> MAHHHHHHHHHHGSTSGSGEQKLISEEDLGSTSGSGDYKDDDDKLTSLYKKAGLENLYFQGMESEMLQSPLLGLGEEDEADLTDWNLPLAFMKKRHCEKIEGSKSLAQSWRMKDRMKTVSVALVLCLNVGVDPPDVVKTTPCARLECWIDPLSMGPQKALETIGANLQKQYENWQPRARYKQSLDPTVDEVKKLCTSLRRNAKEERVLFHYNGHGVPRPTVNGEVWVFNKNYTQYIPLSIYDLQTWMGSPSIFVYDCSNAGLIVKSFKQFALQREQELEVAAINPNHPLAQMPLPPSMKNCIQLAACEATELLPMIPDLPADLFTSCLTTPIKIALRWFCMQKCVSLVPGVTLDLIEKIPGRLNDRRTPLGELNWIFTAITDTIAWNVLPRDLFQKLFRQDLLVASLFRNFLLAERIMRSYNCTPVSSPRLPPTYMHAMWQAWDLAVDICLSQLPTIIEEGTAFRHSPFFAEQLTAFQVWLTMGVENRNPPEQLPIVLQVLLSQVHRLRALDLLGRFLDLGPWAVSLALSVGIFPYVLKLLQSSARELRPLLVFIWAKILAVDSSCQADLVKDNGHKYFLSVLADPYMPAEHRTMTAFILAVIVNSYHTGQEACLQGNLIAICLEQLNDPHPLLRQWVAICLGRIWQNFDSARWCGVRDSAHEKLYSLLSDPIPEVRCAAVFALGTFVGNSAERTDHSTTIDHNVAMMLAQLVSDGSPMVRKELVVALSHLVVQYESNFCTVALQFIEEEKNYALPSPATTEGGSLTPVRDSPCTPRLRSVSSYGNIRAVATARSLNKSLQNLSLTEESGGAVAFSPGNLSTSSSASSTLGSPENEEHILSFETIDKMRRASSYSSLNSLIGVSFNSVYTQIWRVLLHLAADPYPEVSDVAMKVLNSIAYKATVNARPQRVLDTSSLTQSAPASPTNKGVHIHQAGGSPPASSTSSSSLTNDVAKQPVSRDLPSGRPGTTGPAGAQYTPHSHQFPRTRKMFDKGPEQTADDADDAAGHKSFISATVQTGFCDWSARYFAQPVMKIPEEH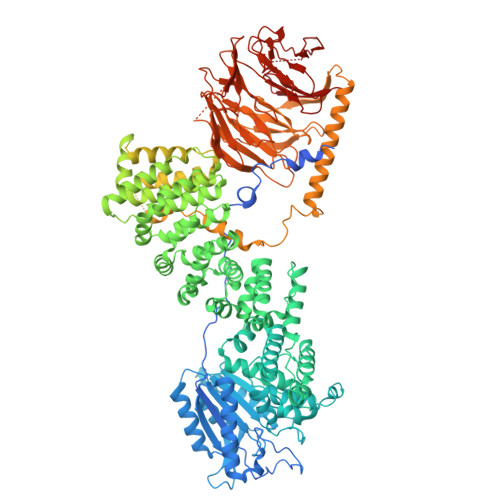DLESQIRKEREWRFLRNSRVRRQAQQVIQKGITRLDDQIFLNRNPGVPSVVKFHPFTPCIAVADKDSICFWDWEKGEKLDYFHNGNPRYTRVTAMEYLNGQDCSLLLTATDDGAIRVWKNFADLEKNPEMVTAWQGLSDMLPTTRGAGMVVDWEQETGLLMSSGDVRIVRIWDTDREMKVQDIPTGADSCVTSLSCDSHRSLIVAGLGDGSIRVYDRRMALSECRVMTYREHTAWVVKASLQKRPDGHIVSVSVNGDVRIFDPRMPESVNVLQIVKGLTALDIHPQADLIACGSVNQFTAIYNSSGELINNIKYYDGFMGQRVGAISCLAFHPHWPHLAVGSNDYYISVYSVEKRVR> GSSPSLEQDDGDEETSVVIVGKISF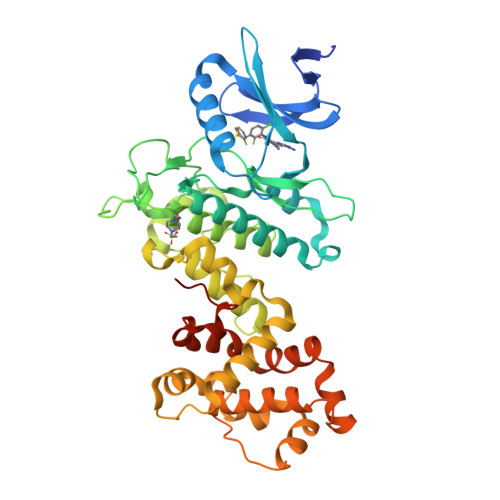CPKDVLGHGAEGTIVYRGMFDNRDVAVKRILPECFSFADREVQLLRESDEHPNVIRYFCTEKDRQFQYIAIELCAATLQEYVEQKDFAHLGLEPITLLQQTTSGLAHLHSLNIVHRNLKPHNILISMPNAHGKIKAMISDFGLCKKLAVGRHSFSRRSGVPGTEGWIAPEMLSEDCKENPTYTVDIFSAGCVFYYVISEGSHPFGKSLQRQANILLGACSLDCLHPEKHEDVIARELIEKMIAMDPQKRPSAKHVLKHPFFWSLEKQLQFFQDVSDRIEKESLDGPIVKQLERGGRAVVKMDWRENITVPLQTDLRKFRTYKGGSVRDLLRAMRNKKHHYRELPAEVRETLGSLPDDFVCYFTSRFPHLLAHTYRAMELCSHERLFQPYYFHEPPEPQPPVTPDALGNS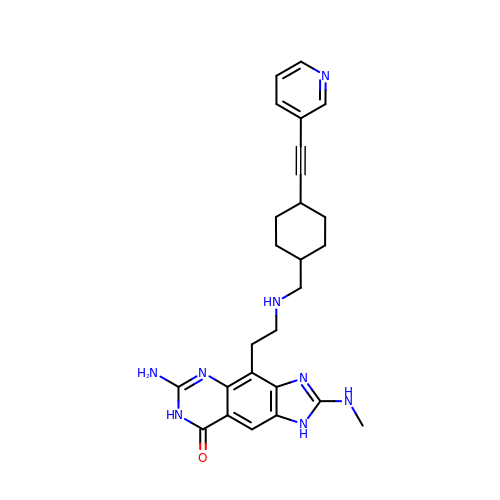6-amino-2-(methylamino)-4-[2-({[trans-4-(pyridin-3-ylethynyl)cyclohexyl]methyl}amino)ethyl]-1,7-dihydro-8H-imidazo[4,5-g]quinazolin-8-one | C26 H30 N8 O | UUKLQSWLBLNLAR-SAABIXHNSA-N>MAFYGKVVKPDETVVPEVKDGYSVIHLSRACLNNPEHEGKIYVQVEDGNGCYNICCLQKNVCEDTPLDIFLMLDNDVKIKTS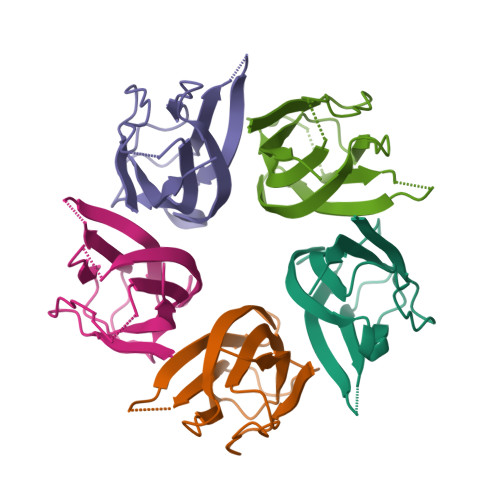GSSNEVHIVGYYEVSFGLEHHHHHH[5x]A newly discovered class of protein organelles called encapsulin nanocompartments have been shown to be involved in microbial iron storage and redox metabolism. Here, we report the structural and mechanistic characterization of the IMEF-system found in Quasibacillus thermotolerans (Qs), an organism that does not encode any ferritins in its genome. We show that this encapsulin-based system self-assembles into a thermostable 42 nm 9.6 MDa protein compartment with a novel T = 4 topology able to mineralize and store an exceptionally large quantity of iron. In contrast to ferritin systems, IMEF encapsulins are two-component systems with the catalytic activity separated from the protein shell.

Through single-particle cryo-EM analysis, we determined the structure of the Qs IMEF encapsulin shell at an overall resolution of 3.85 Å. The IMEF encapsulin self-assembles into a 240-subunit icosahedral compartment with a diameter of 42 nm. The shell is composed of 12 pentameric and 30 hexameric capsomers occupying icosahedral vertices and faces, respectively. The icosahedral asymmetric unit consists of one pentameric and three hexameric monomers. The four capsid proteins of the asymmetric unit adopt different conformations with significant differences found in the E-loop and A-domain. All pores in the IMEF-system are negatively charged on both the exterior and interior surface due to the presence of conserved aspartate, glutamate and asparagine residues. The 3-fold pore forms the largest channel to the IMEF compartment interior and is 7.2 Å wide at its narrowest point, substantially larger than previously reported encapsulin pores. E-loops and P-domains of neighboring capsid monomers arrange head to tail to form interlocking concatenated rings resulting in a non-covalent chainmail topology. Strong TP density is observed for all 180 monomers that are part of 2-fold symmetrical hexameric capsomers while substantially weaker density is found for TPs bound to the 60 pentameric monomers thus revealing higher occupancy and preferential TP binding around 2-fold symmetry axes which can be explained by different binding site conformations and higher local shell mobility. The TP residues TVGSLIQ were tentatively built and refined into the additional density present at hexameric capsomers producing a model with good geometry.

>[4x]MNKSQLYPDSPLTDQDFNQLDQTVIEAARRQLVGRRFIELYGPLGRGMQSVFNDIFMESHEAKMDFQGSFDTEVESSRRVNYTIPMLYKDFVLYWRDLEQSKALDIPIDFSVAANAARDVAFLEDQMIFHGSKEFDIPGLMNVKGRLTHLIGNWYESGNAFQDIVEARNKLLEMNHNGPYALVLSPELYSLLHRVHKDTNVLEIEHVRELITAGVFQSPVLKGKSGVIVNTGRNNLDLAISEDFETAYLGEEGMNHPFRVYETVVLRIKRPAAICTLIDPEE;>[3x]TVGSLIQ>MRSGSHHHHHHRSDITSLYKKAGLENLYFQGSVNPLARFAELVATAGLQSDVQALADSGADDTTLEAQLTQELRLAHDRWGLGLLHLQHSARLIHTDGVPSDIALLVDGAPRAQLSDGARAIAGTYASMQAPGPEGRSEWGILPEGHRVTLRPGLGQLRVLIEDARDFETHWTPGAAQTWTRTWRQGETLAVEVHRPATPATALAKAAWKVITSIKDRTFQRELMERSNQVGMLGALLGARHSGAGDALNQLPEAHFA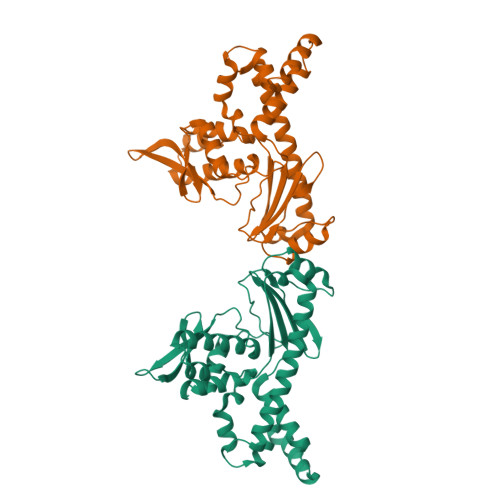VSSAVVRETGREGREVDRWKAMQREATETLDELQKAATRRLAAVLSGGLR[2x]Sugen kinase 223 (SgK223) (also known as Pragmin) and SgK269 (also known as PEAK1) are closely related proteins of 149 and 193 kDa, respectively. Both are classified as pseudokinases due to the substitution of critical residues within highly conserved motifs known to be essential for kinase activity, and both are predicted to function as scaffolds. A recent study found SgK223 and Csk were co-localized at focal adhesions where they regulate cell morphology and motility. Consistent with these findings, SgK223 has emerged as an important regulator of cell morphology, migration and invasion. To gain further insight into the molecular mechanism that drives SgK223 dimerization and oligomerization functions, we solved the crystal structure of the PsK domain of SgK223 and its adjacent regulatory domains.

To fully understand the structural determinants that drive SgK223 dimerization, we solved the crystal structure of a construct (SgK223- αN1-PsK-Cter) that encompasses the PsK domain and the adjacent N- and C-regulatory domains using the multi-wavelength anomalous dispersion method. The structure was refined against native data to 2.95 Å resolution. SgK223 crystallized in space group P43212 with one molecule in the asymmetric unit. Within a monomer, the PsK domain of SgK223 adopts a typical kinase-like fold and the N-terminal helix αN1 directly interacts with the C-terminal helices αJ and αK, while αL helix slides under αI helix of the PsK domain revealing an unusual ‘XL’-shaped helix bundle. While the asymmetric unit contains a monomer, the P43212 crystal form revealed a two-fold symmetric dimer with an extensive buried surface area (BSA) of 1620 Å2. SgK223 dimer formation is mediated by the regulatory helices from the two monomers with the αN1 and the αJ helices from one monomer interacting with the corresponding αJ and αN1 helices from the second monomer to form a unique ‘XX’-shaped four-helix bundle at the ‘core’ of the dimer and positioning the PsK domains peripherally to form the ‘shell’ of the dimer. The most notable feature is the absence of a structured αC helix, a critical feature in bona fide kinases. Instead, in SgK223, the conserved β3 Lys1024 from the YAVK motif makes H-bond interactions with Gln1048 from the loop preceding the β4 strand. The structure of SgK223 clearly demonstrates an absence of an ATP-binding cavity, which is instead occupied by the side chains of residues Tyr1008, Cys1001, Gln1048 and Leu1152. Residues from the αF and αG helices and the end of the A-loop contribute to this interface by intimately packing into a groove created by N-lobe residues Leu994, Trp989, Tyr1009, Ile1025, Phe1054, Val1058 and Val1089 of the PsK domain.

> MHHHHHHHHGSENLYFQGSGSTQLQLHGLLSNISSKEGTYAKLGGLYTQSLARLVAKCEDLFMGGQKKELHFNENNWSLFKLTCNKPCCDSGDAIYYCATCSEDPGSTYAVKICKAPEPKTVSYCSPSVPVHFNIQQDCGHFVASVPSSMLSSPDAPKDPVPALPTHPPAQEQDCVVVITREVPHQTASDFVRDSAASHQAEPEAYERRVCFLLLQLCNGLEHLKEHGIIHRDLCLENLLLVHCTLQAGPGPAPAPAPAPAAAAPPCSSAAPPAGGTLSPAAGPASPEGPREKQLPRLIISNFLKAKQKPGGTPNLQQKKSQARLAPEIVSASQYRKFDEFQTGILIYELLHQPNPFEVRAQLRERDYRQEDLPPLPALSLYSPGLQQLAHLLLEADPIKRIRIGEAKRVLQCLLWGPRRELVQQPGTSEEALCGTLHNWIDMKRALMMMKFAEKAVDRRRGVELEDWLCCQYLASAEPGALLQSLKLLQLL> MRPEVEQELSHVLLTELLAYQFASPVRWIETQDVFLKDYNTERVVEIGPSPTLAGMASRTIKAKYESYDAALSLQRQVLCYAKDTKEIYYTPDPADIAPPIKEEAETSAAATSSSAPAAAAPVSAAPAAAPSGPVAEIPDEPVKAALVLHVLVAHKLKKSLDAVPLSKAIKDLVGGKSTVQNEILGDLGKEFGSTPEKPEDTPLQELAEQFQDTFPGSLGKQTGSLVNRLMSSKMPGGFSLSVARKYLQTRWGLGPGRQDSVLLVALVNEPGARLSSDGEAKEFLDSCAQKYASGAGITLAQAAAGGAGSSGAGGAVIDAEAFEELTKDNRVLARQQLEVLARYLKYDLTKGEKSLVKEKEASSLLQQELDLWAEEHGEIYAQGIKPVFSHLKARTYDSYWNWARQDALSMYFDIIFGKLTDVDRETVSQCIQLMNRSNPTLIKFMQYHIDHCPEYKGETYQLAKSLGQQLIDNCIQVANQDPVYKDISYPTGPHTEVDSKGNIVYKEVNRKSVRKLEQYVFEMSQGGELTKEVQPTIQEDLAKIYEALNKQASTESQLEFNKLYNSLIEFVEKSKEIEVSKSINAVLASKSSDSDRSAEISSLSEKTSIVDPVSGGIPPETVPFLHLKKKLPSGEWVFDRDTSALFLDGLQKGAVNGISYKGKNVLITGAGAGSIGAEVLQGLISGGAKVIVTTSRFSKKVTEYYQDIYARFGAAGSCLIVVPFNQGSKQDVEALIDYIYRDVKDEGLGWDLDAVIPFAAIPEAGIEIDELGSKSELAHRIMLTNLLRLLGEVKKQKFTRAINTRPAQIILPLSPNHGTFGSDGLYSESKLGLETLFNRWYSESWSEQLTVCGAIIGWTRGTGLMSGNNIIAEGLEKLGVRTFSQKEMAFNILGLMTPELTEMCQNGPVVADLNGGLQFIENLREYTAQLRNEIYETSEVRRAVSIETGIETRVVNGENADAPYQKARIEPRANLKFEFPPLKSHKEIQNKAPGLEGLLDLERVIVVTGFGEVSPWGNTRTRWEMEAFGEFSIEGCLEMAWIMGFIKYHNGNLKGKPYTGWIDAKTNEPVEDKDIKKKYEEEILAHAGIRLIEPELFRGYNPEKKELIQEVIIEQDMAPFVTDESTAQQYKLQHEDAVDILKSEESDEYTVTFKKGARLFVPKALRFDRLVAGQIPTGWDAKRYGISEDTISQVDPVTLYALVSTIEALLSAGITDPYEFYKYVHVSEVGNCSGSGMGGVSALRGMFRDRYSDKPVQNDILQESFINTMSAWVNMLLLSSSGPIKTPVGACATAVESVDIGVETILSGKAKICLVGGYDDFQEEGSYEFANMNATSNSLDEFDHGRTPQEMSRPATTTRNGFMEAQGSGTQVIMNAELAIKMGVPIYAIVALTATATDKIGRSVPAPGKGILTTAREHHGSLKTKSPKLDIKYRTRQLNKRKDQIKQWVEDELEYIREEAAELANSDAKFDAVSFVSERTEEVYREATKQVKMAQQEWGNEFWKNDPRIAPLRGALATFNLTVDDLGVASFHGTSTKANDKNESITINKMMQHLGRSEGNPVFGVFQKYLTGHPKGAAGAWMLNGAIQILQTGIVPGNRNADNVDKILEDFEYVLYPSRSIQTDGIKACSVTSFGFGQKGGQAIVVHPDYLFASLDSETFEEYKTKVEARYKSTYRYMHNAIIRNTMFVAKSDPPYTDELEQPVYLDPLARVNNCKKNPSKLVFVNADVQSKQNFVGKSANDTAKVISSLTSDVTSGGKGVGVDVELISAINNENHTFIERNFTENEISYCASAPSSKSSLAGTWSAKEAVFKALGVESKGAGASLKDIEIVRDSKGAPTVVLHGDAKSAASAAGVKNVKVSISHDDVQSVAVAISEF;> MSATSGVVNRPLVLNHGSIESTILIPTTEYHFYQTLLEGFRKSLPQVTEGFADDDEPSSKAELLMKFLGYIVQSGVSNQQEQLAAAKLVLNEFESRFLQGLNLHSYAAILLKSETFPTTLLKIKENLIKNYYLGRALVYLPGQRGLVYPPSALLNAGKSGSAQIYAIFGGQGNTDDYFEELRDIYHIYQGLVSDFVTKAQLKLQELIRTTPETDRIYTQGLDLINWLENKDKTPDQQQLLSIPMSCPLICVIQLCHYIVTCRILGITPGQLRDSLKGTTGHSQGLVTAVVVSSADSWESFEKLALQAVEFMFYIGVRGLQTYPNTSLPPSIVQDSEENAEGTPSPMLSVRDLSYDQLVKFVNETNQHLPEAKHIDISLINGPRNVVLTGPPQSLYGLNLNLRKAKAPSGLDQARIPFSERKLRFSNRFLPIMSPFHSHLLSPSTEKIVADLKKAGVEFSQSSMKLPVFDTYDGKDLRSYSGSIAARLVECITKLRVNWELSTEFNSTHVLDFGPGGASGLGVLTHRNKEGTGSRVIVAGVLDAESEDSEFGYKQEIFESNEKAIKYAPNWLKEYKPKLVKTSAGKIFVDTKFSRLLGRAPLMVPGMTPTTVSPDFVAATLNAGFHTEIAGGGYFAPSIMKAALQRVIDQVTPGTGVGINLIYVNPRMLQWGIPMIKELREQGFPIQSLSIGAGVPSLEVATEYIETLGLAHLGLKPGSIDAVNQVITIAKAHPNFPIVLQWTGGRGGGHHSFEDFHQPILQMYSKIRKCKNIILIAGSGFGSAEDTYPYLTGSWSHQFSYPSMPFDGVLFGSRVMTAKEAKTSPAAKQAIADCTGVDNSQWENTYKKPTGGIITVRSEMGEPIHKIATRGVMLWKELDDTIFTLPKNKMLEAIAKKKDYIIKKLNADYQKPWFAKNEKGTCDLEDMTYKQIAERLVELMYVRKSQRWIDVTLRNFTGKFLRRIEERFATKVGTISLIQNFSQLEEPEKAIDSVFKAYPEAASQLINEEDCDWFLLEAQSPTQKPVPFIPVLDERFEFFFKKDSLWQSEDLEAVVGEDVQRTCILHGPVAAQFSNKVDEPIKDILENIHKGHIKSLVKEVYNGDESKIPVVEYFSSVDSFSDTAIEGVKIERSRNTETFTVTSGNVDNQQWFDLLAGKELSWRRAFITAARLVQGTNFVSNPAHSVLAPSKDLVVKIENGSDAKKTVLTAFQRVRGKYVPAVSLKSIGDLKIKLELIETRTADKSAVALELFYNYKPTDGFAPILEVMEGRNTSIKNFYWKLWFGSSVPVDLDFDANKPISGGEASVSSQAIAEFTHAVGNSCEDFVPRAGRPQLAPMDFAIVLGWKAIMKAIFPKTVDGDILKLVHLSNGYKMFPGADPLKKGDVVSTVAHIRSVVNGETGKTVEVVGVISRDGKPVLEVNSQFFYRGKYQDFGNSFKKTTETPVQVAFKSAKDIAVLKSKEWFHLEKDIDLLN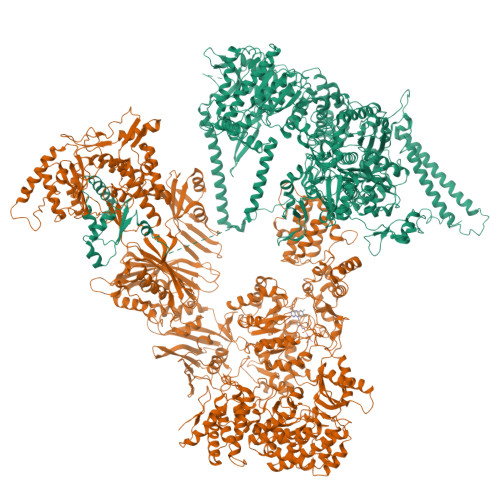QTLTFRCESYVKFKSSTVFASVKTTGQALLELPSKEIIQVAEINYESGSSYGNPVLDYLTRHGSTIEQPIMFENAIPLAQGTELTSKAPGTNETYAAVSGDYNPIHVNKVFASYANLPGTITHGMYSSAAVRALVEQWAAQNVATRVRAFKADFVGMVLPNDELVTHLEHVGMINGRKIIKVETKKVETEEVVLIGEAEIEQPVSTFVFTGQGSQEQGMGMDLYNSSEVAKSVWDRADVHFINNYGFSILDIVKNNPTELTVHFGGAKGRSIRNNYISMMFETVAADGQLKSEKIFKEINEDTISFTFKSPTGLLSATQFTQPALTLMEKASFEDMKSKGLVPSESMFAGHSLGEYSALTSLGDVMPIESLVDVVFYRGMTMQVAVPRDEQGRSNYGMIAVNPSRVSSTFNDSALRFVVEHIAQQTGWLLEIVNYNVENTQYVAAGDLRGLDTLSNVLNVFKIQKIDIVKLQETISLDEVKVHLSEIVDEVSKKSSSKPQPIDLERGFACIPLKGISVPFHSSYLRSGVKPFQTFLCKKIPKSAVKPANLIGKYIPNLTAKPFQLTKEYFEDVYELTKSEKIKHILDHWEEYESS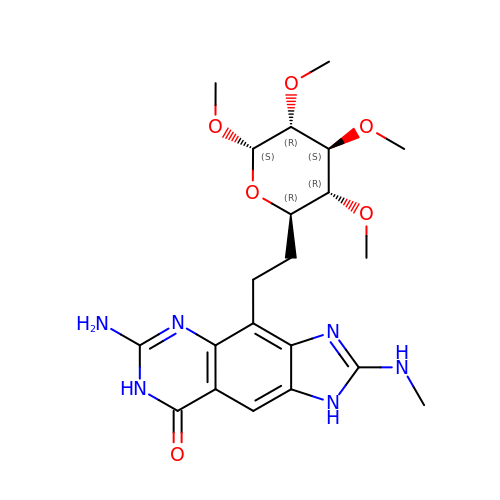6-azanyl-2-(methylamino)-4-[2-[(2~{R},3~{R},4~{S},5~{R},6~{S})-3,4,5,6-tetramethoxyoxan-2-yl]ethyl]-1,7-dihydroimidazo[4,5-g]quinazolin-8-one | C21 H30 N6 O6 | IXUIMEBGCTWFOR-ZIIYPAMZSA-N>SMMSRIAAGDLESSVDDPRSEEDKRFESHIECRKPYKELRLEVGKQRLKYAQEELSNEVLPPPRKMKGLFSQAKISLFYTEEHEIMKFSWRGVTADTRALRRFGFSLAAGRSVWTLEMDAGVLTGRLIRLNDEKWTEMKDDKIVSLIEKFTSNKYWSKVNFPHGMLDLEEIAANSKDFPNMSETDLCFLLHWLNPKKINLADRMLGLSGVQEIK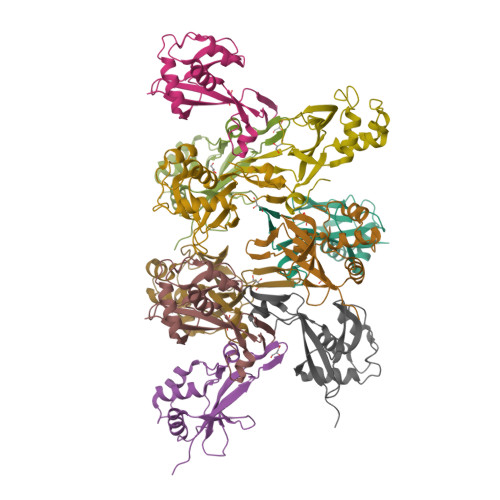EQG[2x]> MSIHFDFKNKQGKELLALNRQWNELSGYRAHAFNESVNMLNNVGETFGVNGANAMQTNMQRVDEMYRLVDSTGTGEDRDWGNQTLLGRLLSQAQTVSIGKKV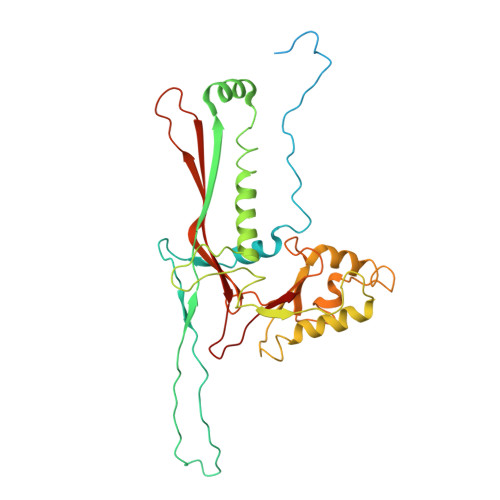IESRRYSEAGRINRSMSGQTDIDMDKTKSSYQKMVIPVFDGAYGRDFRDYEAMRSEMLPALAEDSEEIEFTLLDDVNDYLWNGDAKLKVDTAVWGGLKADASVAAYSLGADLTTATEAQVVAELLALLDVLRITNKKSGPFELYISPQIMSNWQKLAGANTNGFMNIMAAVRALIPEFSVVEADSALQGNQVLCSVVGTRGLHAKIGMMMSSYQVPRVMHNDPYQFVKWFAAGFQSNNSFSGLKSTVYGS> QVYEETAGVRPGEPVVGTGASLSVELGPRLLTSIYDGIQRPLEVIREKTGDFIARGVTAPALPRDKKWHFIPKAKVGDKVVGGDIIGEVPETSIIVHKIMVPPGIEGEIVEIAEEGDYTIEEVIAKVKTPSGEIKELKMYQRWPVRVKRPYKEKLPPEVPLITGQRVIDTFFPQAKGGTAAIPGAFGCGKTVTQHQLAKWSDAQVVIYIGCGERGNEMTDVLEEFPKLKDPKTGKPLMERTVLIANTSNMPVAAREASIYTGITIAEYFRDMGYDVALMADSTSRWAEALREISGRLEEMPGEEGYPAYLASKLAEFYERAGRVVTLGSDYRVGSVSVIGAVSPPGGDFSEPVVQNTLR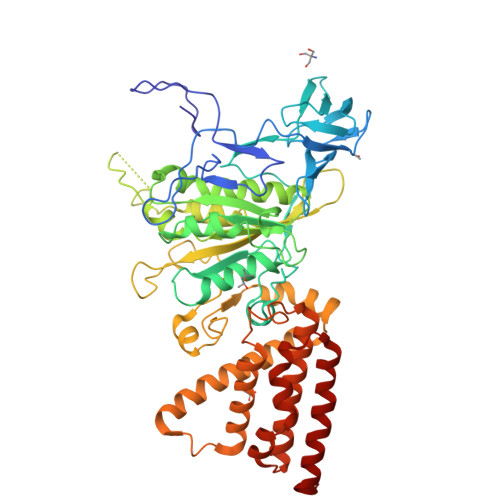VVKVFWALDADLARRRHFPAINWLTSYSLYVDAVKDWWHKNIDPEWKAMRDKAMALLQKESELQEIVRIVGPDALPERERAILLVARMLREDYLQQDAFDEVDTYCPPEKQVTMMRVLLNFYDKTMEAINRGVPLEEIAKLPVREEIGRMKFERDVSKIRSLIDKTNEQFEELFKKYGA> ESFADMMKHGLTEADVGITKFVSSHQGFSGILKERYSDFVVHEIGKDGRISHLNDLSIPVDEEDPSEDIFTVLTAEEKQRLEELQLFKNKETSVAIEVIEDTKEKRTIIHQAIKSLFPGLETKTEDREGKKYIVAYHAAGKKALANPRKHSWPKSRGSYCHFVLYKENKDTMDAINVLSKYLRVKPNIFSYMGTKDKRAITVQEIAV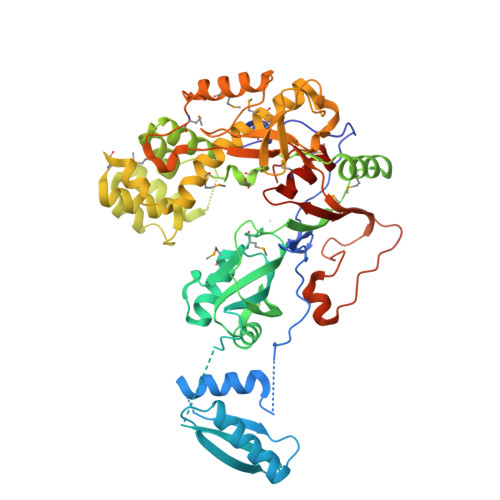LKITAQRLAHLNKCLMNFKLGNFSYQKNPLKLGELQGNHFTVVLRNITGTDDQVQQAMNSLKEIGFINYYGMQRFGTTAVPTYQVGRAILQNSWTEVMDLILKPRSGAEKGYLVKCREEWAKTKDPTAALRKLPVKRCVEGQLLRGLSKYGMKNIVSAFGIIPRNNRLMYIHSYQSYVWNNMVSKRIEDYGLKPVPGDLVLKGATATYIEEDDVNNYSIHDVVMPLPGFDVIYPKHKIQEAYREMLTADNLDIDNMRHKIRDYSLSGAYRKIIIRPQNVSWEVVAYDDPKIPLFNTDVDNLEGKTPPVFASEGKYRALKMDFSLPPSTYATMAIREVLKMDTSIKNQTQLNTTWLR> MAHHHHHHMTSVGLIWAQSTSGVIGRDGGIPWRLPEDLAHFKRLTMGHTVVMGRRTWDSLPAAHRPLPGRRNVVVTRQTGLVAHGAQVVGS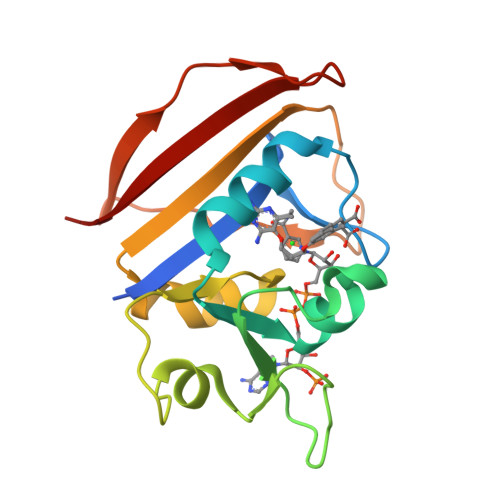LEQALCPAEPDAATWVIGGAQIYALALPLANRCEVTEVDVDLPPEDEDALAPVLDQTWAGTSGEWLVSRSGLRYRMHSYRRL(2R,3R,4R,5R)-4-hydroxy-2,5-bis(hydroxymethyl)pyrrolidin-3-yl 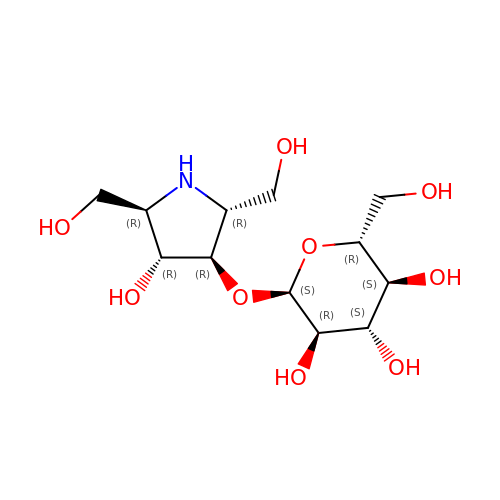alpha-D-glucopyranoside | C12 H23 N O9 | AZDBETUGBOOBRU-BBFNFCGLSA-N ToxR is a transmembrane transcription factor involved in the regulation of numerous genes, not only virulence associated, and can function as an activator, co-activator and repressor. ToxS is built of a periplasmic, a transmembrane and a short cytoplasmic region. The periplasmic domain of ToxS (ToxSp) interacts with the periplasmic domain of ToxR (ToxRp) forming a stable heterodimer (ToxRSp; Gubensäk et al., 2021b) thereby protecting ToxR from periplasmic proteolysis and enhancing its activity. Located at the inner membrane, ToxR and ToxS react to environmental stimuli like bile acid, thereby inducing survival strategies for example bile resistance and virulence regulation.

ToxRSp crystal structure was determined by molecular replacement using an AlphaFold model as template. ToxRp in the complex has an αß fold which is formed by an α-helix flanked by an anti-parallel hairpin and a three-stranded anti-parallel ß-sheet, followed by a C-terminal helix. ToxSp forms a lipocalin-like fold consisting of an eight-stranded ß-barrel stabilized by intermolecular H-bond network and flanked by two α-helices located at the openings of the barrel. However, ToxSp ß8 contacts only the first three residues of nine residues long ToxSp ß1. ToxRp ß5 is positioned into this gap and forms main chain H-bonds with remaining ToxSp ß1 residues. The residue Arg281 located in ToxRp ß5 forms an intermolecular salt bridge with Asp142 of ToxSp α2, which restricts the opening of the barrel. When bound to ToxSp, the unstructured region of the C-terminus of ToxRp performs a disorder to order transition, by forming two additional structural elements: short α helix 2 and ß strand 5. The newly formed short α helix 2 contacts the turn between ToxSp ß1 and ß2, as well as residues Leu45ToxSp and Ile46ToxSp located at the C-terminal part of ToxSp ß1 thus increasing the interaction interface and further stabilizing the fold. L33 forms central hydrophobic interactions with apolar residues of ToxSp ß strands stabilizing the core of the barrel. The ToxRS complex exposes a bile binding pocket inside ToxS lipocalin-like barrel that is only properly built via stabilization by newly formed structural elements of ToxR.

> MRGSHHHHHHGSPSQTSFKPLTVVDGVAVNMPNNHPDLSNWLPSIELCVKKYNEKHTGGLKPIEVIATGGQNNQLTLNYIHSPEVSGENITLRIVANPNDAIKVCE;> MGSSHHHHHHSQDPNSDFKLEQVLTSREWQSKMVSLIKTNSNRPAMGPLSRVDVTSNVKYLPNGTYLRVSIVKLFSDDNSAESVINISEFGEWDISDNYLLVTPVEFKDISSNQSKDFTDEQLQLITQLFKMDAQQSRRVDIVNERTILFTSLSHGSTVLFSNS> AKLSCKICGYIYDEDEGDPDNGISPGTKFEDLPDDWVCP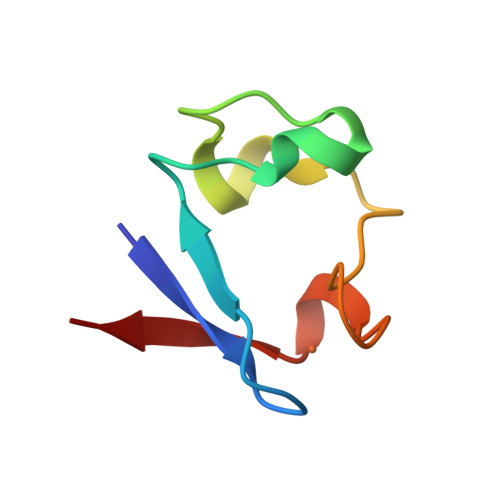LCGAPKSEFERIE>SNAMAEIKITPEELERIAGNFKNAAGEAQSQINRLEGDINSLEGQWAGATQAKFRGQFIQSKQA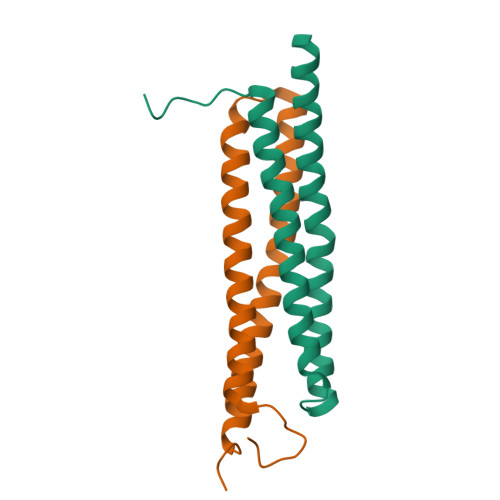MQQYIPILEGISTDLKRIADKFRNTDNAY[4x]>[4x]MHHHHHHMKEIATEYSFIKYTELELDDNGSIKQLSIPNKYNVIYAIAIND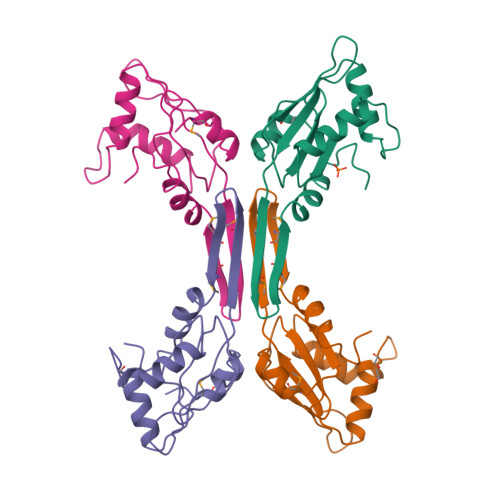ELVYIGKTKNLRKRINYYRTAINRKDKTSDSTKSALIHSALKEGSKVEFYARQCFNLSMTNELGTMTIATIDLEAPLFIKLFNPPWNIQHKKK F420 is a low-potential redox cofactor used by diverse bacteria and archaea. In mycobacteria, this cofactor has multiple roles, including adaptation to redox stress, cell wall biosynthesis, and activation of the clinical antitubercular prodrugs pretomanid and delamanid. To determine the structural basis of dehydro-F420-0 production, we solved high-resolution crystal structures of the enzyme responsible (FbiA) in apo-, substrate-, and product-bound forms. The crystal structure of FbiA shows that this enzyme employs a flexible active site to capture Fo and EPPG, precisely positioning them for catalysis.

Similarly, FbiA crystals were soaked with Fo and GDP, individually or in combination, and structures of substrate-bound FbiA were determined. In the GDP and Fo-bound structure, the coordination of Ca2+ is analogous to the GDP-only structure. However, the glycerol molecule and one of the H2O molecules observed in the GDP-only structure are displaced by the ribosyl chain of Fo, resulting in a coordination number of six with octahedral geometry. The terminal hydroxyl group of Fo is significantly closer to the Ca2+ ion (2.6 Å) and to the β-phosphate of GDP (2.8 Å from O and 3.0 Å from P) than the coordinating hydroxyl of glycerol, which is not within the bonding distance of GDP. These bond distances between the hydroxyl of Fo and GDP, as well as the central orientation of the hydroxyl of Fo toward the β-phosphate of GDP, place it in an ideal position to act as the acceptor substrate for the transfer of PEP catalyzed by FbiA. Determination of the fully resolved FbiA substrate complex, in the presence of a single catalytic metal ion, provides a clear picture of the mechanism of catalysis of this enzyme. In this structure, the terminal hydroxyl group of Fo is ideally positioned for nucleophilic attack of the β-phosphate of EPPG, strongly suggesting that DH-F420-0 biosynthesis occurs through direct transfer of PEP to Fo, via a pentavalent phosphate intermediate that is stabilized by the catalytic metal ion. As no acidic side chains are present in proximity of the terminal hydroxyl of Fo in our structure of FbiA, it is likely that deprotonation of this group for nucleophilic attack is EPPG induced, possibly by the PEP carboxyl moiety.

>MKITVLVGGVGGARFLLGVQNLLGLGSFADGPSKHELTAVVNIGDDAWMHGVRICPDLDTCMYTLGGGIDPDRGWGHRNETWNAKEELAAYGVQPDWFGLGDRDLATHLVRSQMLRAGYPLSQVTEALCKRWQPGARLLPASDERSETHVVITDPTDGERRAIHFQEWWVRYRAKVPTHSFAYVGADQATAGPGVVEAIGDADIVLLAPSNPVVSIGPILQIPGIRGALRSTSAPVIGYSPIIAGKPLRGMADECLKVIGVESTSQAVGEFFGARAGTGLLDGWLVHEGDHAQIEGVKVKAVPLLMTDPEATAAMVRAGLDLAGVSL[2x]>[2x]TDKLTSLRQYTTVVADTGDIAAMKLYQPQDATTNPSLILNAAQIPEYRKLIDDAVAWAKQQSNDRAQQIVDATDKLAVNIGLEILKLVPGRISTAVDARL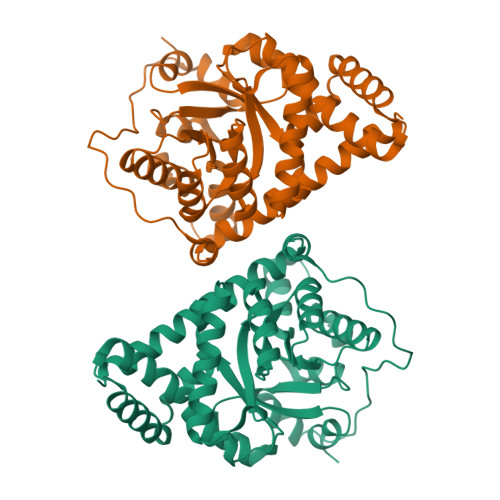SYDTEASIAKAKRLIKLYNDAGISNDRILIKLASTWQGIRAAEQLEKEGINCNLTLLFSFAQARACAEAGVFLISPFVGRILDWYKANTDKKEYAPAEDPGVVSVSEIYQYYKEHGYETVVMGASFRNIGEILELAGCDRLTIAPALLKELAESEGAIERKLSYTGEVKARPARITESEFLWQHNQDPMAVDKLAEGIRKFAIDQEKLEKMIGDLL>MNPVAFIREKREGKKHRREDLEAFLLGYLRDEVPDYQVSAWLMAAFLRGLDPEETLWLTETMARSGKVLDLSGLPHPVDKHSSGGVGDKVSLVVGPILAASGCTFAKMSGRGLAHTGGTIDKLESVPGWRGEMTEAEFLERARRVGLVIAAQSPDLAPLDGKLYALRDVTATVESVPLIASSIMSKKLAAGARSIVLDVKVGRGAFMKTLEEARLLAKTMVAIGQGAGRRVRALLTSMEAPLGRAVGNAIEVREAIEALKGEGPGDLLEVALALAEEALRLEGLDPALARKALEGGAALEKFRAFLEAQGGDPRAVEDFSLLPLAEEHPLRAEREGVVREVDAYKVGLAVLALGGGRKRKGEPIDHGVGVYLLKKPGDR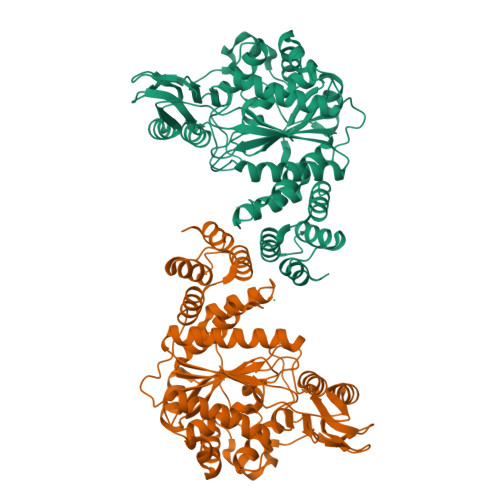VERGEALALVYHRRRGLEEALGHLREAYALGEEAHPAPLVLEAI[2x]>[4x]MTQQIGVIGLAVMGKNLAWNIESRGYSVSVFNRSSEKTDLMVEESKGKNIHPTYSLEEFVNSLEKPRKILLMVQAGKATDATIDSLLPLLDDGDILIDGGNTNYQDTIRRNKALAQ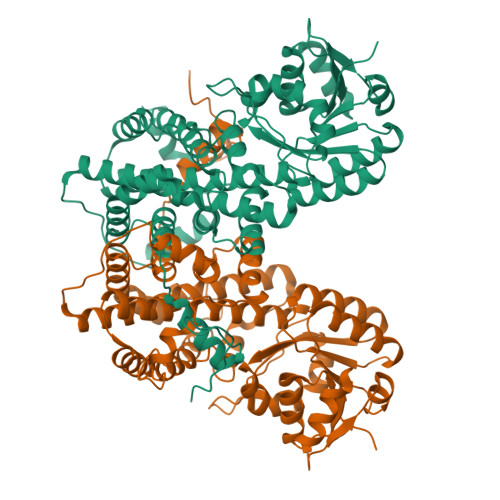SAINFIGMGVSGGEIGALTGPSLMPGGQEEAYNKVADILDAIAAKAKDGASCVTYIGPNGAGHYVKMVHNGIEYADMQLIAESYAMMKELLGMSHEDIAQTFKDWNAGELESYLIEITGDIFMKLDENKEALVEKILDTAGQKGTGKWTSINALELGIPLTIITESVFARFISSIKEERVNASKELNGPKASFDGDKKDFLEKIRKALYMSKICSYAQGFAQMRKASEDNEWNLKLGDLAMIWREGCIIRAQFLQKIKDAYDNNPGLQNLLLDPYFKNIVTEYQDALRDVVATGVQNGVPTPGFSSSINYYDSYRAADLPANLIQAQRDYFGAHTYERKDKEGVFHTQWIEE3-methylbenzohydrazide | C8 H10 N2 O | 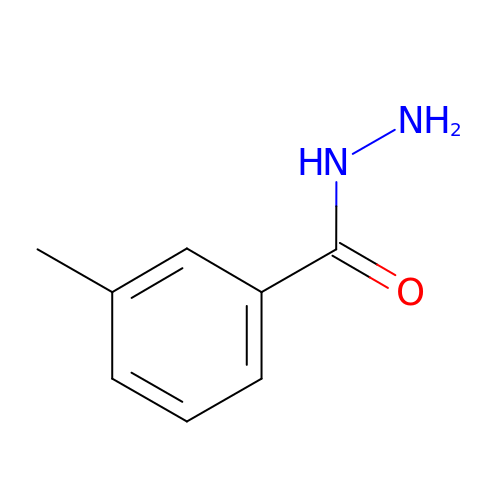XFNNAMBYJSQXKF-UHFFFAOYSA-N> GSKKLAEYKCNTNTAIELKLVRFPEDLENDIRTFFPEYTHQLFGDDETAFGYKGLKILLYYIAGSLSTMFRVEYASKVDENFDCVEADDVEGKIRQIIPPGFCTNTNDFLSLLEKEVDFKPFGTLLHTYSVLSPTGGENFTFQIYKADMTCRGFREYHERLQTFLMWFIETASFIDVDDERWHYFLVFEKYNKDGATLFATVGYMTVYNYYVYPDKTRPRVSQMLILTPFQGQGHGAQLLETVHRYYTEFPTVLDITAEDPSK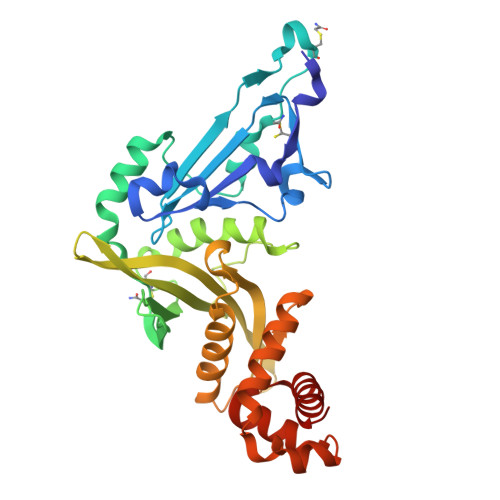SYVKLRDFVLVKLCQDLPCFSREKLMQGFNEDMAIEAQQKFKINKQHARRVYEILRLLVTD>HHHHHHHHVPEAFLLFSRRADIRRISLETNNNNVAIPLTGVKEASALDFDVTDNRIYWTDISLKTISRAFMNGSALEHVVEFGLDYPEGMAVDWLGKNLYWADTGTNRIEVSKLDGQHRQVLVWKDLDSPRALALDPAEGFMYWTEWGGKPKIDRAAMDGSERTTLVPNVGRANGLTIDYAKRRLYWTDLDTNLIESSNMLGLNREVIADDLPHPFGLTQYQDYIYWTDWSRRSIERANKTSGQNRTIIQGHLDYVMDILVFHSSRQSGWNECASSNGHCSHLCLAVPVGGFVCGCPAHYSLN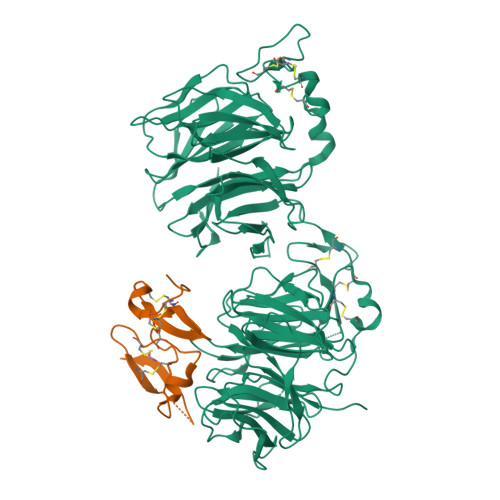ADNRTCSAPTTFLLFSQKSAINRMVIDEQQSPDIILPIHSLRNVRAIDYDPLDKQLYWIDSRQNMIRKAQEDGSQGFTVVVSSVPSQNLEIQPYDLSIDIYSRYIYWTCEATNVINVTRLDGRSVGVVLKGEQDRPRAIVVNPEKGYMYFTNLQERSPKIERAALDGTEREVLFFSGLSKPIALALDSRLGKLFWADSDLRRIESSDLSGANRIVLEDSNILQPVGLTVFENWLYWIDKQQQMIEKIDMTGREGRTKVQARIAQLSDIHAVKELNLQEYRQHPCAQDNGGCSHICLVKGDGTTRCSCPMHLVLLQDELSC[2x];> GPGSGQEGSVCLRSSDCASGLCCARHFWSKICKPVLKEGQVCTKHRRKGSHGLEIFQRCYCGEGLSCRIQKDHHQASNSSRLHTCQRH>MALTQVETEIVPVSVDGETLTVEAVRRVAEERATVDVPAESIAKAQKSREIFEGIAEQNIPIYGVTTGYGEMIYMQVDKSKEVELQTNLVRSHSAGVGPLFAEDEARAIVAARLNTLAKGHSAVRPIILERLAQYLNEGITPAIPEIGSLGASGDLAPLSHVASTLIGEGYVLRDGRPVETAQVLAERGI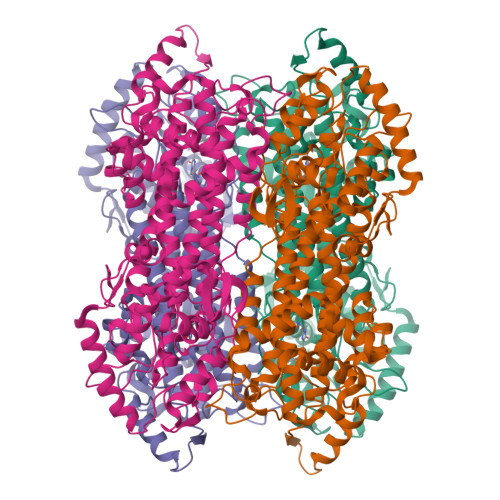EPLELRFKEGLALINGTSGMTGLGSLVVGRALEQAQQAEIVTALLIEAVRGSTSPFLAEGHDIARPHEGQIDTAANMRALMRGSGLTVEHADLRRELQKDKEAGKDVQRSEIYLQKAYSLRAIPQVVGAVRDTLYHARHKLRIELNSANDNPLFFEGKEIFHGANFHGQPIAFAMDFVTIALTQLGVLAERQINRVLNRHLSYGLPEFLVSGDPGLHSGFAGAQYPATALVAENRTIGPASTQSVPSNGDNQDVVSMGLISARNARRVLSNNNKILAVEYLAAAQAVDISGRFDGLSPAAKATYEAVRRLVPTLGVDRYMADDIELVADALSRGEFLRAIARETDIQLR[2x]>MLEMATVEPETTPTPNPPTTEEEKTESNQEVANPEHYIKHPLQNRWALWFFKNDKSKTWQANLRLISKFDTVEDFWALYNHIQLSSNLMPGCDYSLFKDGIEPMWEDEKNKRGGRWLITLNKQQRRSDLDRFWLETLLCLIGESFDDYSDDVCGAVVNVRAKGDKIAIWTTECENREAVTHIGRVYKE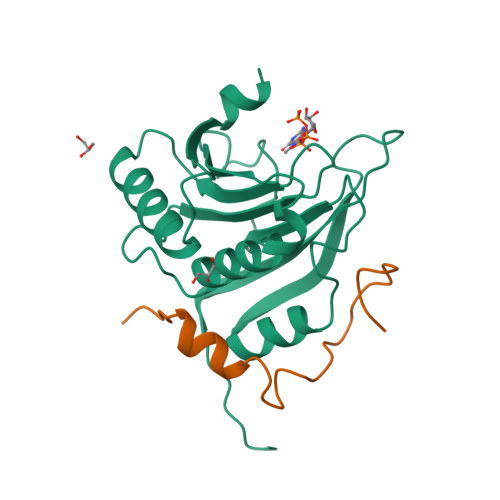RLGLPPKIVIGYQSHADTATKSGSTTKNRFVV[2x];>GPHMQKYEYKSDQWKPLNLEEKKRYDREFLLGFQFIFASMQKPEGLPHISDVVLDKANKTPLRPLD[2x]> MMIRINLLPVRAVKKREMGRQVLVLFAVVLIGAGVANYLWYDDRQSELEAHQAGVASTKARIAELEKIIGEVKNINTRKAEVEKKLAV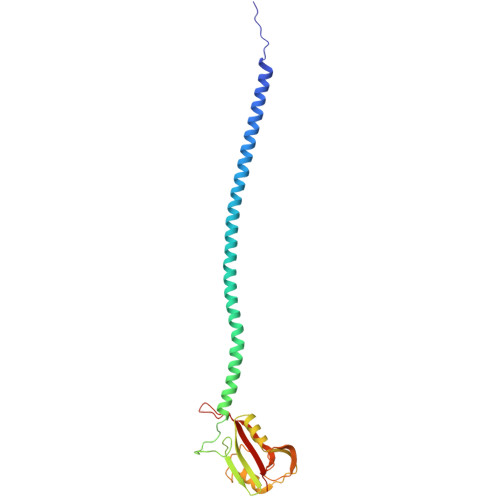LDALRKGRSGPVRMMDALASATPKKVWVKTFSENNNAVSIDGSAVSHDEVAEFMRGLNGVVWTPKGMGRLVDRRRDSKTARVEMLTSDATIEEFPEAQVSPFFKNIDLQTAKQVGGAQVGVPILVEFKITMTSNYAI> MGSDKIH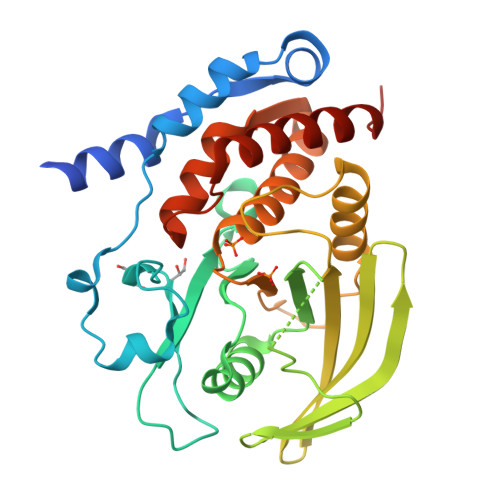HHHHHMNTPREVTLHFLRTAGHPLTRWALQRQPPSPKQLEEEFLKIPSNFVSPEDLDIPGHASKDRYKTILPNPQSRVCLGRAQSQEDGDYINANYIRGYDGKEKVYIATQGPMPNTVSDFWEMVWQEEVSLIVMLTQLREGKEKCVHYWPTEEETYGPFQIRIQDMKECPEYTVRQLTIQYQEERRSVKHILFSAWPAHQTPESAGPLLRLVAEVEESPETAAHPGPIVVHCSAGIGRTGCFIATRIGCQQLKARGEVDILGIVCQLRLDRGGMIQTAEQYQFLHHTLALYAGQLPEEPSP[(2~{R},3~{S},4~{S},5~{R})-5-[3-(4-octyl-1,2,3-triazol-1-yl)propyl]-3,4-bis(oxidanyl)oxan-2-yl]methyl ~{N}-[(2~{S})-2-azanyl-4-methyl-pentanoyl]sulfamate | C25 H47 N5 O7 S | 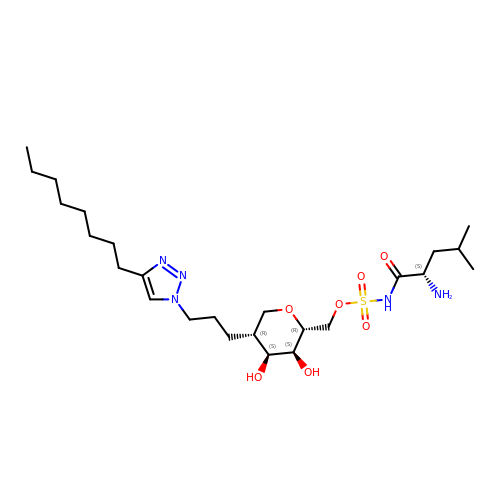KJHVCACMAXYEPW-MENZVKOBSA-N>MACVNEPSPKLQKLDRNGIHGDSSPSPFFKVKKLSEKAVIPTRGSPLSAGYDLSSAVDSKVPARGKALIPTDLSIAVPEGTYARIAPRSGLAWKHSIDVGAGVIDADYRGPVGVILFNHSDADFEVKFG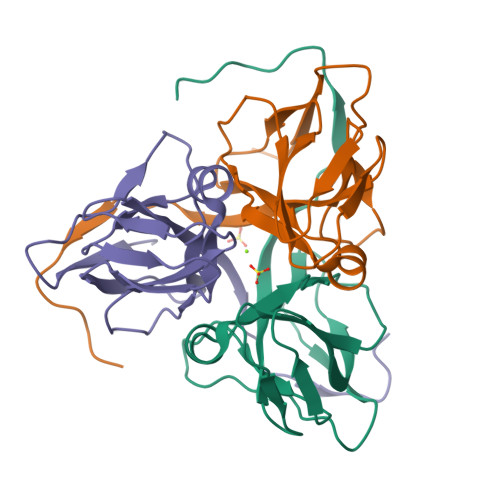DRIAQLIIEKIVTPDVVEVDDLDETVRGDGGFGSTGV[3x]>MTNQDRPMKSMSESKCYKNRQVFPQDTNHHHTMFGGTLMANIDEIAAITAMKHAGAQVVTASTDSVDFLKPIKTGDILQYVAMVSYAGTSSMEVVVQIRIDDVFNNKHDLAALSYLTFVALDDEGKPKHVPGVYPEDDVEKWFYDTAPQRVERRKARRIESKQTIEYL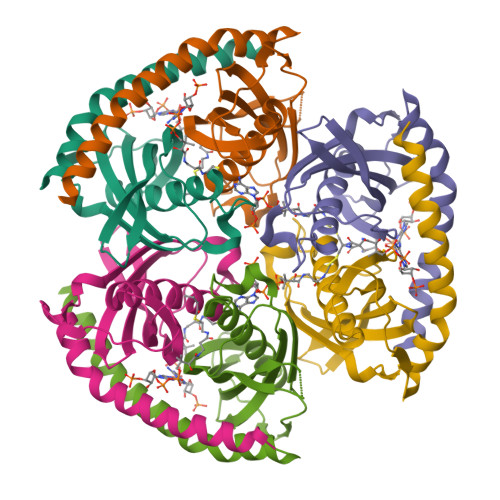AQAQHIRD[3x]> MSMSTSTEVIAHHWAFAIFLIVAIGLCCLMLVGGWFLGGRARARSKNV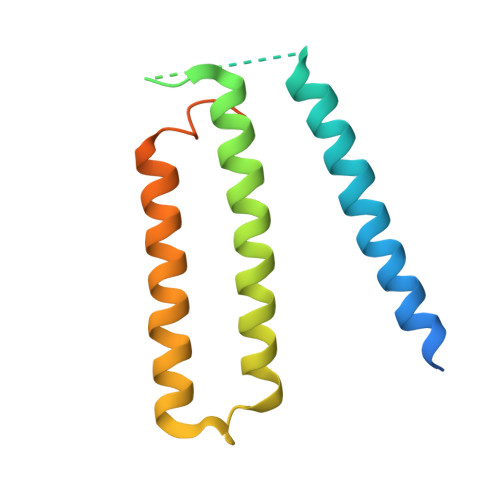PFESGIDSVGSARLRLSAKFYLVAMFFVIFDVEALYLFAWSTSIRESGWVGFVEAAIFIFVLLAGLVYLVRIGALDWTPARSRRERMNPETNSIANRQR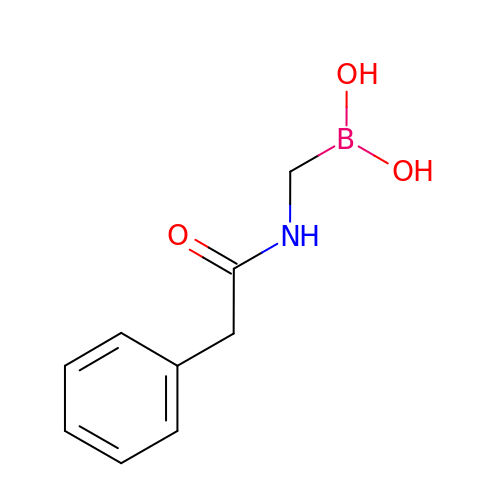PHENYLACETAMIDOMETHYL BORONIC ACID | C9 H12 B N O3 | WPZJZIUTEZTIJI-UHFFFAOYSA-N> IVGGTSASAGDFPFIVSISRNGGPWCGGSLLNANTVLTAAHCVSGYAQSGFQI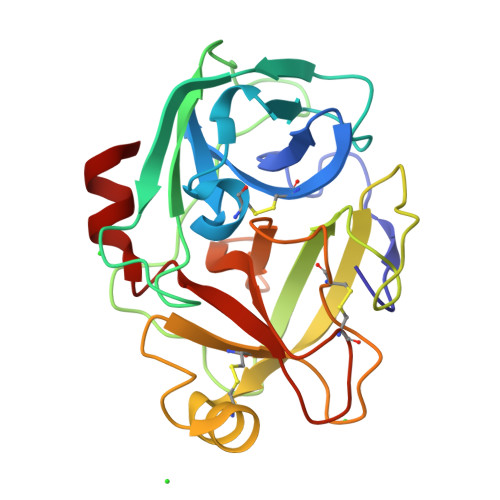RAGSLSRTSGGITSSLSSVRVHPSYSGNNNDLAILKLSTSIPSGGNIGYARLAASGSDPVAGSSATVAGWGATSEGGSSTPVNLLKVTVPIVSRATCRAQYGTSAITNQMFCAGVSSGGKDSCQGDSGGPIVDSSNTLIGAVSWGNGCARPNYSGVYASVGALRSFIDTYA2-{[(2E)-3-(naphthalen-2-yl)but-2-enoyl]amino}benzoic acid | C21 H17 N O3 | 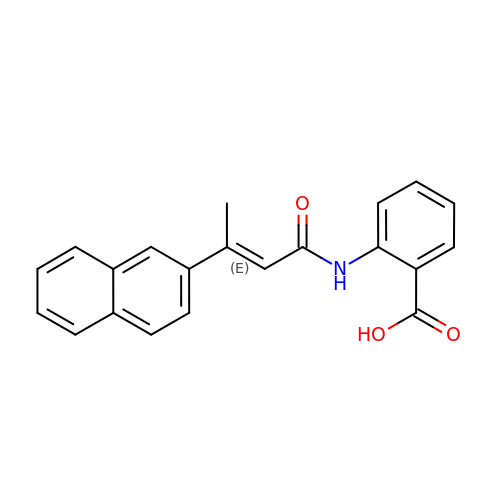PGFQXGLPJUCTOI-WYMLVPIESA-N>MEITPSDVIKTLPRQEFSLVFQKVKEMEKTGAHIINLGQGNPDLPTPPHIVEALREASLNPSFHGYGPFRGYPFLKEAIAAFYKREYGVTINPETEVALFGGGKAGLYVLTQCLLNPGDIALVPNPGYPEYLSGITMARAELYEMPLYEENGYLPDFEKIDPAVLEKAKLMFLNYPNNPTGAVADAAFYAKAAAFAKEHNIHLIHDFAYGAFEFD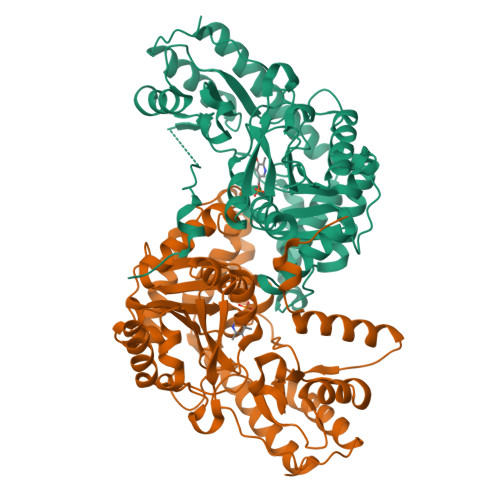QKPASFLEAEDAKTVGAELYSFSKTFNMAGWRMAFAVGNEKIIQAVNEFQDHVFVGMFGGLQQAASAALSGDPEHTESLKRIYKERIDFFTALCEKELGWKMEKPKGTFYVWAEIPNTFETSHQFSDYLLEHAHVVVTPGEIFGSNGKRHVRISMVSKQEDLREFVTRIQKLNLPFGSLQETSR[2x]> SRCTHLENRDFVTGVQGTTRLTLVLELGGCVTVTADGKPSLDVWLDSIYQESPAQTREYCLHAKLTGTKVAARCPTMGPATLPEEHQSGTVCKRDQSDRGWGNHCGLFGKGSIVTCVKFTCEDKKKATGHVYDVNKITYTIKVEPHTGEFVAANETHSGRKSASFTVSSEKTILTLGDYGDVSLLCRVASGVDLAQTVVLALDKTHEHLPTAWQVHRDWFNDLALPWKHDGAEAWNEAGRLVEFGTPHAVKMDVFNLGDQTGVLLKSLAGVPVASIEGTKYHLKSGHVTCEVGLEKLKMKGLTYTVCDKTKFTWKRAPTDSGHDTVVMEVGFSGTRPCRIPVRAVAHGVPEVNVAMLITPNPTMENNGGGFIEMQLPPGDNIIYVGDLNHQW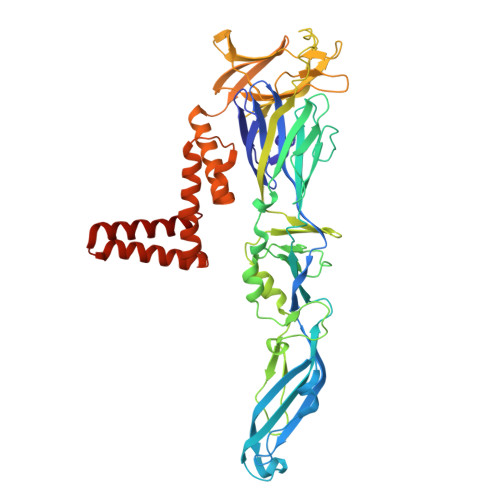FQKGSSIGRVLQKTRKGIERLTVLGEHAWDFGSVGGVMTSIGRAMHTVLGGAFNTLLGGVGFLPKILLGVAMAWLGLNMRNPTLSMGFLLSGGLVLAMTLGVGA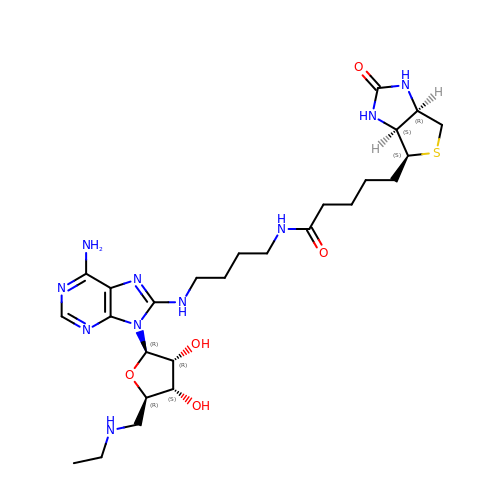5'-DEOXY-5'-(ETHYLAMINO)-8-{[4-({5-[(3AS,4S,6AR)-2-OXOHEXAHYDRO-1H-THIENO[3,4-D]IMIDAZOL-4-YL]PENTANOYL}AMINO)BUTYL]AMINO}ADENOSINE | C26 H42 N10 O5 S | GZOCMSGHLSHCGU-DGWADGOTSA-N>[2x]CACGCG;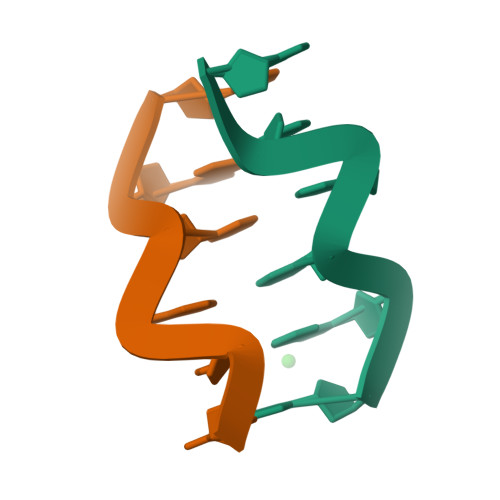>[2x]CGCGTG> GMSESCILFFVKYPEPGKVKTRLGEVVGNDKAAMLYRHFVQDMLQGLARLHADLHICYVPGDADLPEKFKAWLGPQHMFAAQQGLDLGERMKHAMQKAFDDGYDRVVLMGSDIPDYPCELVQKALNDLQHYDAAIGPAFDGGYYLIGFRKDSFCPDVFDGIRWGEADVYQPTVEKMRRARLEVLQLPDWNDVDTVWDLNVLYRTNKNSSFRRSSTYALLRENDALIRQYDIDLPGMAPVEK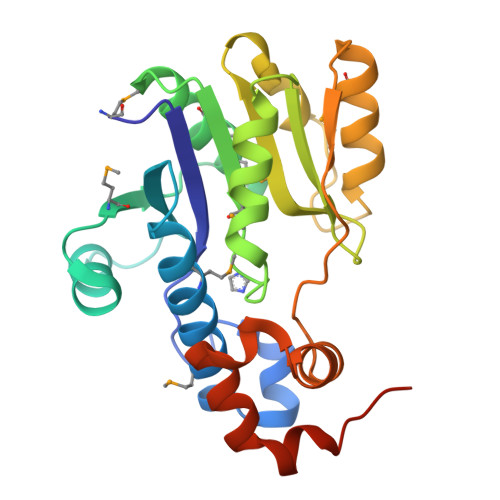E> MSDKDSKNTPQVPEKLGLSRRGFLGASAVTGAAVAATALGGAVMTRESWAQAVKESKQKIHVGPGELDDYYGFWSGGHQGEVRVLGVPSMRELMRIPVFNVDSATGWGLTNESRHIMGD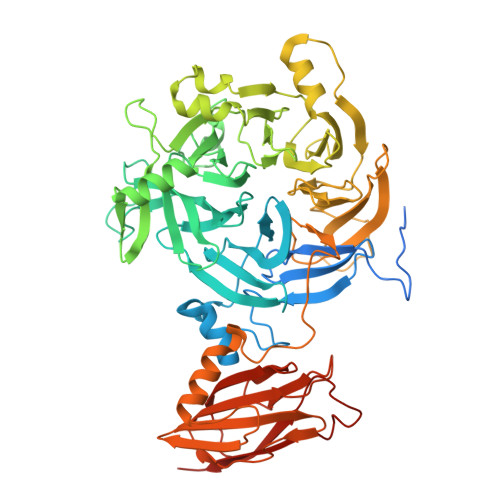SAKFLNGDCHHPHISMTDGKYDGKYLFINDKANSRVARIRLDIMKCDKMITVPNVQAIHGLRLQKVPHTKYVFANAEFIIPHPNDGKVFDLQDENSYTMYNAIDAETMEMAFQVIVDGNLDNTDADYTGRFAAATCYNSEKAFDLGGMMRNERDWVVVFDIHAVEAAVKAGDFITLGDSKTPVLDGRKKDGKDSKFTRYVPVPKNPHGCNTSSDGKYFIAAGKLSPTCSMIAIDKLPDLFAGKLADPRDVIVGEPELGLGPLHTTFDGRGNAYTTLFIDSQVVKWNMEEAVRAYKGEKVNYIKQKLDVHYQPGHLHASLCETNEADGKWLVALSKFSKDRFLPVGPLHPENDQLIDISGDEMKLVHDGPTFAEPHDCIMARRDQIKTKKIWDRNDPFFAPTVEMAKKDGINLDTDNKVIRDGNKVRVYMTSMAPAFGVQEFTVKQGDEVTVTITNIDQIEDVSHGFVVVNHGVSMEISPQQTSSITFVADKPGLHWYYCSWFCHALHMEMVGRMMVEPAWSHPQFEK> ATFISVQLKKTSEVDLAKPLVKFIQQTYPSGGEEQAQYCRAAEELSKLRRAAVGRPLDKHEGALETLLRYYDQICSIEPKFPFSENQICLTFTWKDAFDKGSLFGGSVKLALASLGYEKSCVLFNCAALASQIAAEQNLDNDEGLKIAAKHYQFASGAFLHIKETVLSALSREPTVDISPDTVGTLSLIMLAQAQEVFFLKATRDKMKDAIIAKLANQAADYFGDAFKQCQYKDTLPKEVFPVLAAKHCIMQANAEYHQSILAKQQYYFGEEIARLQHAAELIKTVASRYDEYVNVKDFSDKINRALAAAKKDNDFIYHDRVPDLKDLDPIGKATLVKSTPVNVPISQKFTDLFEKMVPVSVQQSLAAYNQRKADLVNRSIAQMREATTLANGVLASLNLPAAIEDVSGDTVPQSILTKSRSVIEQGGIQTVDQLIKELPELLQRNREILDESLRLLDEEEATDNDLRAKFKERWQRTPSNELYKPLRAEGTNFRTVLDKAVQADGQVKECYQSHRDTIVLLCKPEPELNAAIPSANPAKTMQGSEVVNVLKSLLSNLDEVKKEREGLENDLKSVNFDMTSKFLTALAQDGV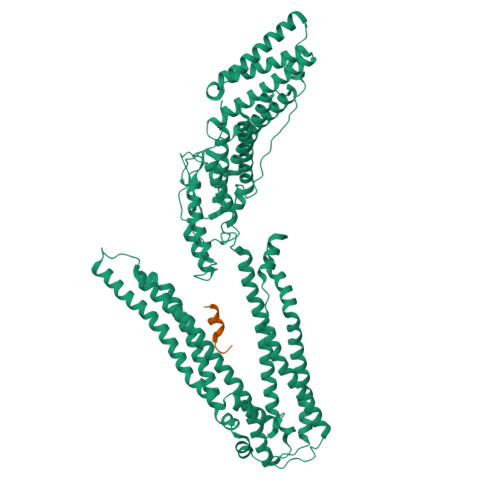INEEALSVTELDRVYGGLTTKVQESLKKQEGLLKNIQVSHQEFSKMKQSNNEANLREEVLKNLATAYDNFVELVANLKEGTKFYNELTEILVRFQNKCSDIVFAR;> ELYPLTSLRSL> MEDKKIVIMPCKCAPSRQLV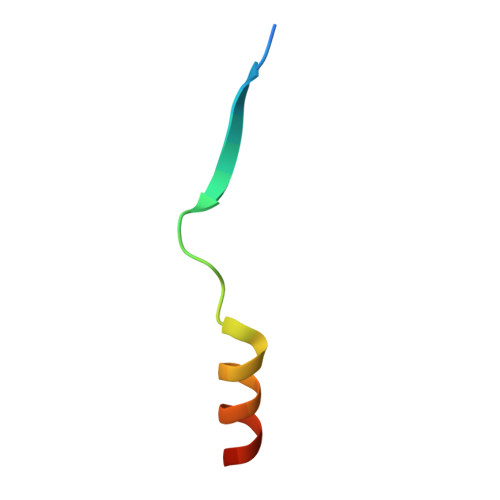QVWLQAKE(3R,4R)-1-[(4-AMINO-5H-PYRROLO[3,2-D]PYRIMIDIN-7-YL)METHYL]-4-(HYDROXYMETHYL)PYRROLIDIN-3-OL | C12 H17 N5 O2 | 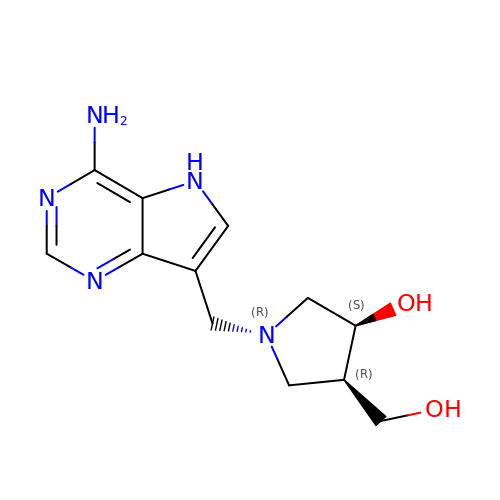HYYXEHQHMXTTFP-BDAKNGLRSA-N>MGSDKIHHHHHHENLYFQGMQLLKELCSIHAPSGNEEPLKDFILEYIRSNAGSWSYQPVIYADNDLQDCIVLVFGNPRTAVFAHMDSIGFTVSYNNHLHPIGSPSAKEGYRLVGKDSNGDIEGVLKIVDEEWMLETDRLIDRGTEVTFKPDFREEGDFILTPYLDDRLGVWTALELAKTLEHGIIAFTCWEEHGGGSVAYLARWIYETFHVKQSLICDITWVTEGVEAGKGVAISMRDRMIPRKKYVNRIIEL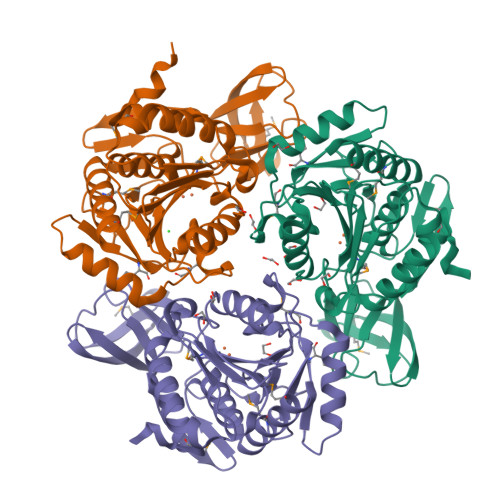ARQTDIPFQLEVEGAGASDGRELQLSPYPWDWCFIGAPEKDAHTPNECVHKKDIESMVGLYKYLMEKL[3x]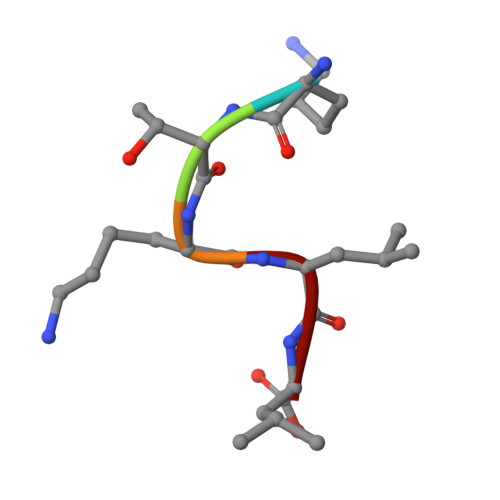> KTKLL> GEFGDEDLEELCPVCGDKVSGYHYGLLTCESCKGFFKRTVQNNKRYTCIENQNCQIDKTQRKRCPYCRFQKCLSVGMKLEAVRADRMR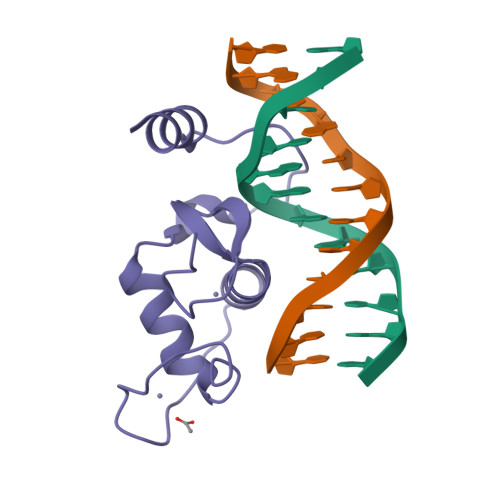GGRNKFGPMYKRDRALKQQKKALIR> MKVEELIIDGFKSYATRTVITDWDPQFNAITGLNGSGKSNILDAICFVLGIASMSTVRASSLQDLIYKRGQAGVTKASVTIVFDNTDKSNSPIGFTNSPQISVTRQVVLGGTSKYLINGHRAPQQSVLQLFQSVQLNINNPNFLIMQGKITKVLNMKPSEILSLIEEAAGTKMFEDRREKAERTMSKKETKLQENRTLLTEEIEPKLEKLRNEKRMFLEFQSTQTDLEKTERIVVSYEYYNIKHKHTSIRETLENGETRMKMLNEFVKKTSEEIDSLNEDVEEIKLQKEKELHKEGTISKLENKENGLLNEISRLKTSLSIKVENLNDTTEKSKALESEIASSSAKLIEKKSAYANTEKDYKMVQEQLSKQRDLYKRKEELVSTLTTGISSTGAADGGYNAQLAKAKTELNEVSLAIKKSSMKMELLKKELLTIEPKLKEATKDNELNVKHVKQCQETCDKLRARLVEYGFDPSRIKDLKQREDKLKSHYYQTCKNSEYLKRRVTNLEFNYTKPYPNFEASFVHGVVGQLFQIDNDNIRYATALQTCAGGRLFNVVVQDSQTATQLLERGRLRKRVTIIPLDKIYTRPISSQVLDLAKKIAPGKVELAINLIRFDESITKAMEFIFGNSLICEDPETAKKITFHPKIRARSITLQGDVYDPEGTLSGGSRNTSESLLVDIQKYNQIQKQIETIQADLNHVTEELQTQYATSQKTKTIQSDLNLSLHKLDLAKRNLDANPSSQIIARNEEILRDIGECENEIKTKQMSLKKCQEEVSTIEKDMKEYDSDKGSKLNELKKELKLLAKELEEQESESERKYDLFQNLELETEQLSSELDSNKTLLHNHLKSIESLKLENSDLEGKIRGVEDDLVTVQTELNEEKKRLMDIDDELNELETLIKKKQDEKKSSELELQKLVHDLNKYKSNTNNMEKIIEDLRQKHEFLEDFDLVRNIVKQNEGIDLDTYRERSKQLNEKFQELRKKVNPNIMNMIENVEKKEAALKTMIKTIEKDKMKIQETISKLNEYKRETLVKTWEKVTLDFGNIFADLLPNSFAKLVPCEGKDVTQGLEVKVKLGNIWKESLIELSGGQRSLIALSLIMALLQFRPAPMYILDEVDAALDLSHT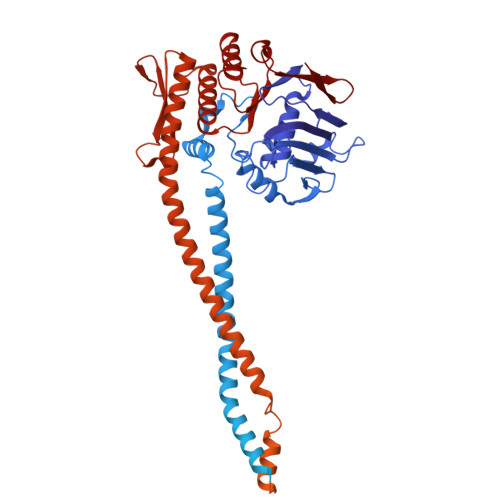QNIGHLIKTRFKGSQFIVVSLKEGMFANANRVFRTRFQDGTSVVSIM>[4x]MSLINARLIAFEDQWVPALNAPLKQAILADSQDAQLAAAMTYSVLAGGKRLRPLLTVATMQSLGVTFVPERHWRPVMALELLHTYSLIHDDLPAMDNDALRRGEPTNHVKFGAGMATLAGDGLLTLAFQWLTATDLPATMQAALVQALATAAGPSGMVAGQAKDIQSEHVNLPLSQLRVLHKEKTGALLHYAVQAGLILGQAPEAQWPAYLQFADAFGLAFQIYDDILDVVSSPAEMGKATQKDADEAKN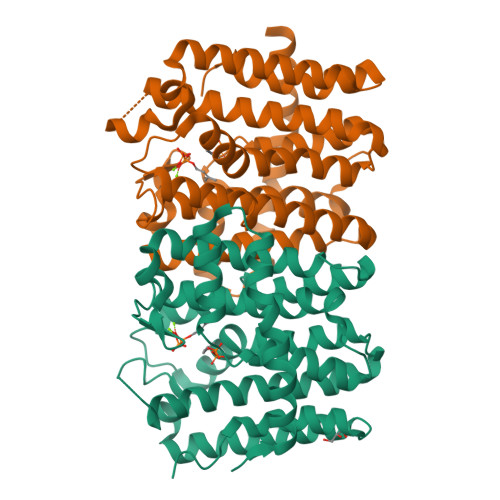TYPGKLGLIGANQALIDTIHSGQAALQGLPTSTQRDDLAAFFSYFDTERVNEGHHHHHH>MLGAVEGPRWKQAEDIRDIYDFRDVLGTGAFSEVILAEDKRTQKLVAIKCIAKEALEGKEGSMENEIAVLHKIKHPNIVALDDIYESGGHLYLIMQLVSGGELFDRIVEKGFYTERDASRLIFQVLDAVKYLHDLGIVHRDLKPENLLYYSLDEDSKIMISDFGLSKMEDPGSVLSTACGTPGYVAPEVLAQKPYSKAVDCWSIGVIAYILLCGYPPFYDENDAKLFEQILKAEYEFDSPYWDDISDSAKDFIRHLMEKDPEKRFTCEQALQHPWIAGDTALDKNIHQSVSEQIKKNFAKSKWKQAFNATAVVRH[2x]

When activated, CaM binds to and stimulates the activities of a family of Ca2+/CaM-dependent serine/threonine protein kinases (CaMKs), thereby regulating their functions. However, the regulation mechanism of CaMKI remains elusive. Here we report four crystal structures of three truncation variants of human CaMKIα, namely CaMKI320 (residues 1–320), CaMKI315 (residues 1–315), and CaMKI293 (residues 1–293), which correspond to the aforementioned three truncation forms of CaMKI, respectively. The catalytic core of CaMKI takes a canonical bilobate architecture, with the N-terminal lobe (N lobe) consisting of five antiparallel β-strands and a prominent helix named helix αC and the C-terminal lobe (C lobe) comprised primarily of α-helices.

CaMKI315 containing the autoinhibition segment cannot be activated by CaM as the CaM-binding segment is incomplete. The CaMKI315-ATP structure is very similar to the CaMKI320-ATP structure and also adopts an inactive conformation. The bound ATP shows evident electron density and maintains similar interactions with the enzyme as in the CaMKI320-ATP complex; however, the phosphate groups of ATP have a much higher average B factor and no Mg2+ was observed in the electron density. In addition, in the CaMKI320-ATP and CaMKI315-ATP structures which are crystallized in another space group (P63), two pseudo two-fold symmetry-related molecules are juxtaposed head to tail in a similar way as in the apo CaMKI320. However, helix αT is largely disordered in one molecule and completely disordered in the other, although the hydrophobic cluster at the interface is partially maintained. Although the CaMKI320-ATP and CaMKI315-ATP complexes show substantial differences from the apo CaMKI320 in the activation segment and the nucleotide-binding site, in all three structures helix αR1 (residues 287–297) of the autoinhibitory segment interlocks with helices αD and αF, and the surrounding structure elements including the αD-αE loop and helix αE adopt essentially identical conformations. Superposition of these structures with Akt/PKB-GSK3β shows that the residues at the P(-5) and P(-6) positions of the substrate peptide would collide with the C-terminal part of helix αR1, suggesting that helix αR1 might exert the inhibitory function via occlusion of part of the substrate-binding site. ATP binding can induce conformational changes at the nucleotide-binding site and the activation segment, leading to the formation of an inactive, pre-CaM binding state which is represented by the CaMKI320-ATP and CaMKI315-ATP structures (pre-CaM binding state). In this state, the activation segment is largely disordered and its restraint on helix αC is alleviated. Nevertheless, helix αC remains in an inactive conformation and the catalytic site is only partially assembled.>GS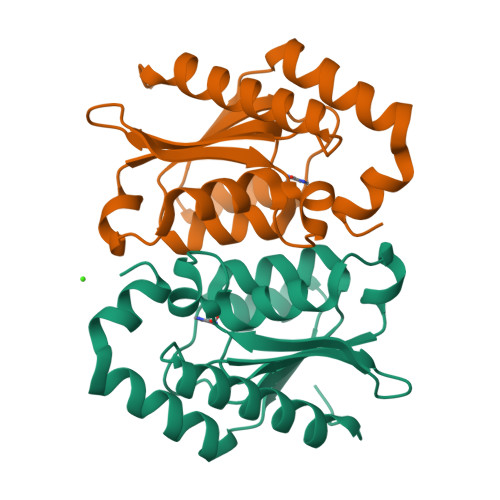SMVTGGMASKWDQKGMDIAYEEALLGYKEGGVPIGGCLINNKDGSVLGRGHNMRFQKGSATLHGEISTLENCGRLEGKVYKDTTLYTTLSPCEMCTGAIIMYGIPRCVIGENVNFKSKGEKYLQTRGHEVVVVDDERCKKLMKQFIDERPQDWFEDIGE[2x]> MEPAGRFTKVAAAVADSVVTIESVSDQEGMQGSGVIVDGRGYIVTNNHVISEAANNPSQFKTTVVFNDGKEVPANLVGRDPKTD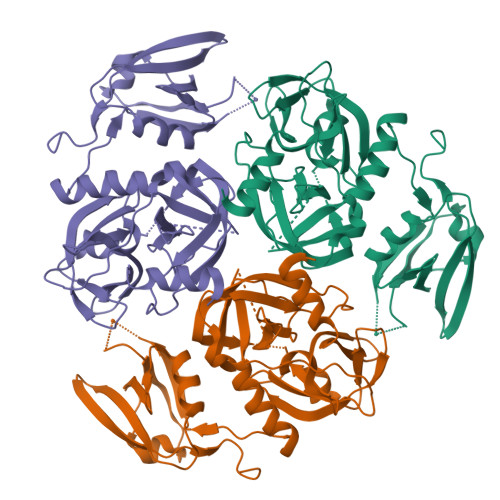LAVLKVDNVDNLTVARLGDSSKVRVGDEVLAVGAPLGLRSTVTQGIVSALHRPVPLSGEGADTDTVIDAIQTDASINHGNSGGPLIDMDAQVIGINTAGKSLSDSASGLGFAIPVNEMKLVANSLIKDGKIVHPTLGISTRSVSNAIASGAQVANVKAGSPAQKGGILENDVIVKVGNRAVADSDEFVVAVRQLAIGQDAPIEVVREGRHVTLTVKPDPDSTLEHHHHHH> PISPIETVPVKLKPGMDGPKVKQWPLTEEKIKALVEICTEMEKEGKISKIGPENPYNTPVFAIKKKDSTKWRKLVDFRELNKRTQDFWEVQLGIPHPAGLKKKKSVTVLDVGDAYFSVPLDEDFRKYTAFTIPSINNETPGIRYQYNVLPQGWKGSPAIFQSSMTKILEPFRKQNPDIVIYQYMDDLYVGSDLEIGQHRTKIEELRQHLLRWGLTTPDKKHQKEPPFLWMGYELHPDKWTVQPIVLPEKDSWTVNDICKLVGKLNWASQIYPGIKVRQLS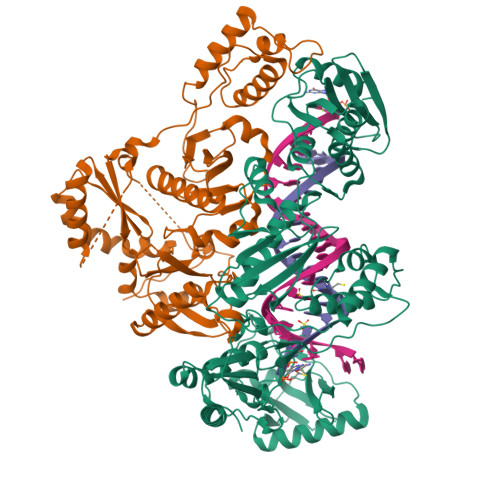KLLRGTKALTEVIPLTEEAELELAENREILKEPVHGVYYDPSKDLIAEIQKQGQGQWTYQIYQEPFKNLKTGKYARMRGAHTNDVKQLTEAVQKITTESIVIWGKTPKFKLPIQKETWETWWTEYWQATWIPEWEFVNTPPLVKLWYQLEKEPIVGAETFYVDGAANRETKLGKAGYVTNRGRQKVVTLTDTTNQKTELQAIYLALQDSGLEVNIVTDSQYALGIIQAQPDQSESELVNQIIEQLIKKEKVYLAWVPAHKGIGGNEQVDKLVSAGIRKVL;> MGSSHHHHHHSSPISPIETVPVKLKPGMDGPKVKQWPLTEEKIKALVEICTEMEKEGKISKIGPENPYNTPVFAIKKKDSTKWRKLVDFRELNKRTQDFWEVQLGIPHPAGLKKKKSVTVLDVGDAYFSVPLDEDFRKYTAFTIPSINNETPGIRYQYNVLPQGWKGSPAIFQSSMTKILEPFRKQNPDIVIYQYMDDLYVGSDLEIGQHRTKIEELRQHLLRWGLTTPDKKHQKEPPFLWMGYELHPDKWTVQPIVLPEKDSWTVNDIQKLVGKLNWASQIYPGIKVRQLSKLLRGTKALTEVIPLTEEAELELAENREILKEPVHGVYYDPSKDLIAEIQKQGQGQWTYQIYQEPFKNLKTGKYARMRGAHTNDVKQLTEAVQKITTESIVIWGKTPKFKLPIQKETWETWWTEYWQATWIPEWEFVNTPPLVKLWYQLEKEPIVGAETF>[4x]GSVGNPVEARRWLRQARANFSAARNDLHKNANEWVCFKCYLSTKLALIAADYAVRGKSDKDVKPTALAQKIEE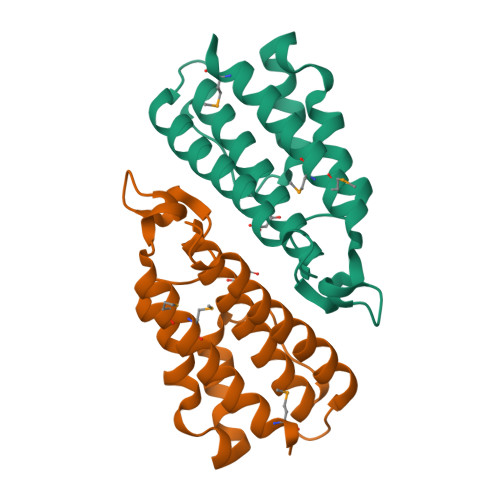YSQQLEGLTNDVHTLEAYGVDSLKTRYPDLLPFPQIPNDRFTSEVAMRVMECTACIIIKLENFMQQKV Solution and crystal data are reported for DNA 18-mers with sequences related to those of bacterial noncoding single-stranded DNA segments called repetitive extragenic palindromes (REPs). REPs are DNA segments of about 30 nucleotides in length that occur frequently in some bacterial species. The center of the duplex is formed by two successive T–T mismatches.

In this study, we focus on two REP-related oligonucleotide sequences called Hpar-18 and Chom-18. The crystal structures of all three oligonucleotides, Chom-18, Chom-18Br and Hpar-18, were determined using highly anisotropic data at a relatively low resolution of worse than 2.6 Å. Experimental phasing was necessary because no molecular model was available. The subsequent refinement unequivocally established that all three 18-mers form antiparallel double helices in the crystal phase. The structures are highly similar: the calculated r.m.s.d. between all 365 non-H atoms of Chom-18 and Hpar-18 is 1.0 Å and the r.m.s.d. between Chom-18 and Chom-18Br is 0.24 Å. The crystal structures contain one central and one (in Hpar-18 and Chom-18Br) or two (in Chom-18) peripheral Sr2+ cations. In all three structures the central Sr2+ links the two O4 atoms of the symmetry-related mismatched thymines T9–T9*. In all cases the crystallization solutions contained Na+, a quadruplex-inducing metal, but also the quadruplex-breaking Mg2+ (in Chom-18 and Chom-18Br) and Li+ (in Hpar-18). In both the Chom-18 and Chom-18Br structures, all but two central steps are assigned to NtC classes, while in Hpar-18 two additional steps, 4–5 and 12–13, cannot be assigned and are formally assigned NtC class NANT.

> GGTGGGGCTTGCCCCACC> MPQSDGISNLHRIALRFPKEGGGYDMYRFKVNPENYTIDSPQRTTAIKTKSDIVIEDYGKDIEVINFTGTTGFRPVREADGLKTGKQKMEELQSRVSEYAMQGGSGNVSGSYLQFFNFTDDSYYKVHLAPQGLKITRSKDEPLLFRYEITLVVIGSLTE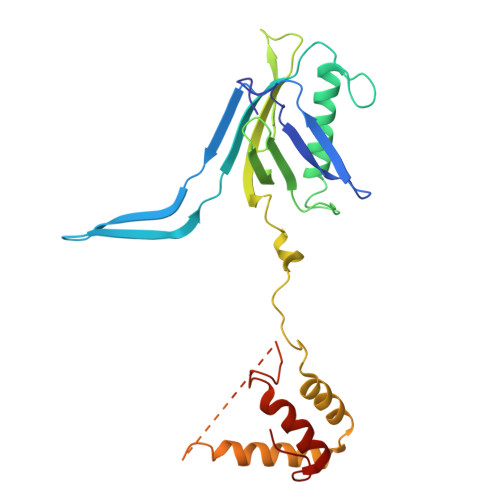ADRSAVTTEEFGNVKPNASQRVDEGIKELDKNARKTRDRNNQEISRRENTIPKSTGDNTNEGNRLKQSFPSSSIYNPRQSTNGLKGNIDNMALIIGYGDGGVSS>[5x]SNAMSSLSKEAELVHQALLAR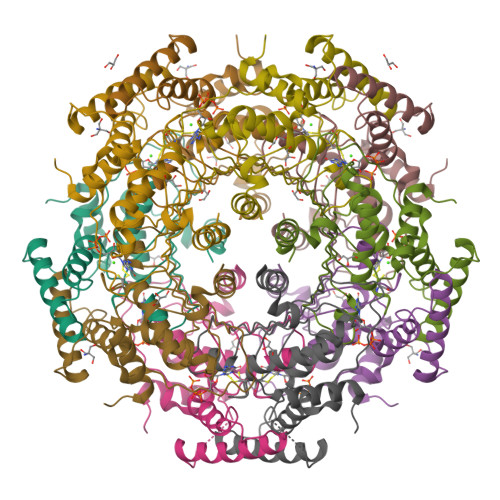GLETPLRKPELDAETRKTRIQAHMTEVMHLLNLDLTDDSLADTPRRIAKMYVDEIFSGLDYENFPKITLIQNKMKVDEMVTVRDITLTSTCEHHFVTIDGKATVAYIPKDSVIGLSKINRIVQFFAQRPQVQERLTQQILLALQTLLGTNNVAVSIDAVHYCVKARGIRDATSATTTTSLGGLFKSSQNTRQEFLRAVRHHG> QDGGWSHWSPWSSCSVTCGDGVITRIRLCNSPSPQMNGKPCEGEARETKACKKDACPINGGWGPWSPWDIC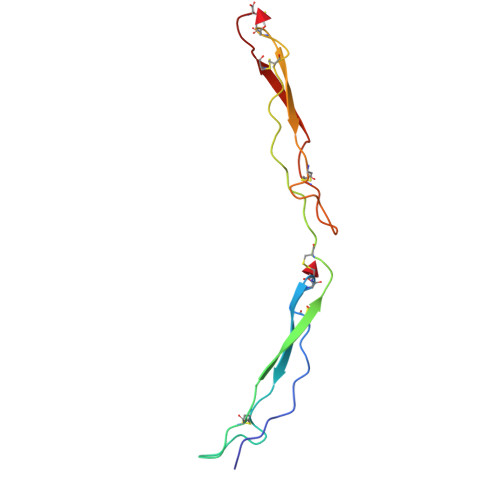SVTCGGGVQKRSRLCNNPTPQFGGKDCVGDVTENQICNKQDC> MDETDPILTQKNWDGTATYFQSSDEHGFSMYYKPQVGFVGDPMPFYDPVAKDFKVMYLQDYRPNPEATYHPIFGVATKDGATYES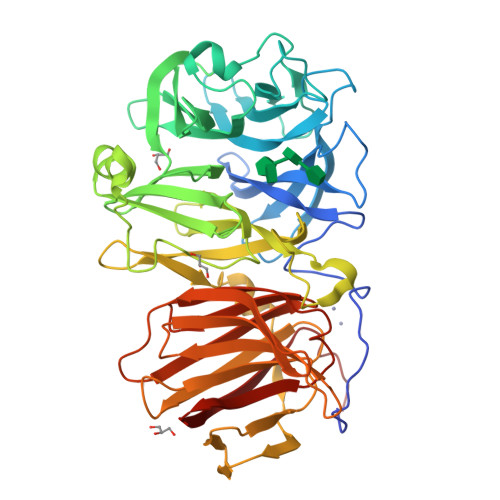LGELISCGGRDEQDAAIGTGGTIYNPADKLYYTFYTGNKFKPSSDQNAQVVMVATSPDFKTWTKNRTFYLKGDTYGYDKNDFRDPFLFQTEDGVYHMLIATRKNGKGHIAEFTSADLKEWESAGTFMTMMWDRFYACPDVFKMGDWWYLIYSEQASFMRKVQYFKGRTLEDLKATTANDAGIWPDNREGMLDSRAFYAGKTASDGTNRYIWGWCPTRAGNDNGNVGDVEPEWAGNLVAQRLIQHEDGTLTLGVPDAIDRKYTSAQEVKVMAKDGNMIESGKTYTLGEGASVIFNRLKVHNKISFTVKTASNTDRFGISFVRGTDSASWYSIHVNADEGKANFEKDGDDAKYLFDNKFNIPADNEYRVTIYSDQSVCVTYINDQLSFTNRIYQMQKNPWSLCCYKGEITVSDVQVSTYHHHHHH>[3x]GGGSIKEITETTQLIVKHLAHNGEEYSEVVKEISEEMEKKGLS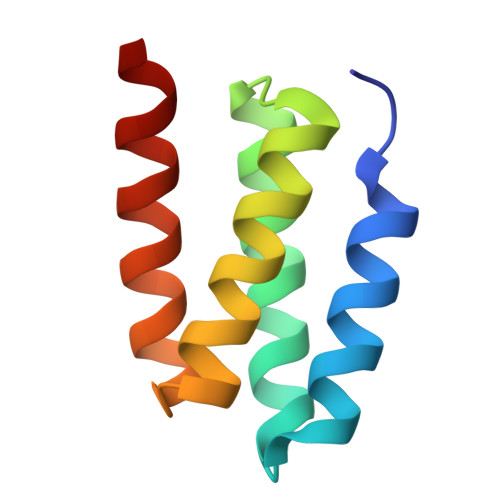KEQVILLLIHFLLLSLVKGLSPETTKLLMKELIKELEKIK> MKKLLLILMSVALFSTAAQAARIKDVAQVAGVRSNQLVGYGLVSGLPGTGEANPFTEQSFAAMLQNFGIQMPPGTKPKIKNVAAVMVTAELPPFSKPGQQVDVTVSSIGSAKSLRGGTLLQTFLKGLDGQVYAVAQGNLVVSGFSAEGADGSKIVGNNPTVGLISSGATVEREIPNPFGRGDYITFNLLESDFTTAQRMADAVNNFLGPQMASAVDATSVRVRAPRDVSQRVAFL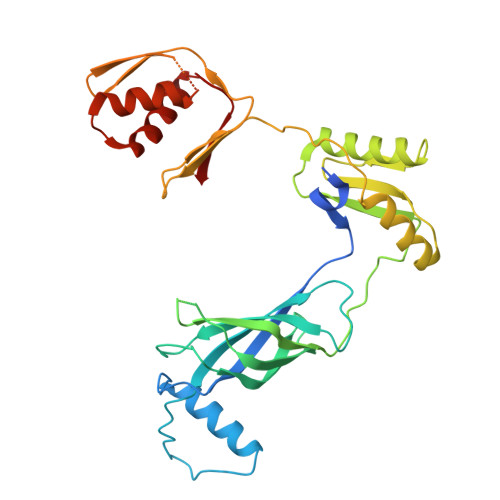SAIENLEFDPADGAAKIIVNSRTGTIVVGKHVRLKPAAVTHGGMTVAIKENLNVSQPNGFSGGQTVVVPDSDIEVSEEQGKMFKFEPGLTLDDLVRAVNQVGAAPSDLMAILQALKQAGAIEGQLIII> MVYSYTEKKRIRKDFGKRPQVLDVPYLLSIQLDSFQKFIEQDPEGQYGLEAAFRSVFPIQSYSGNSELQYVSYRLGEPVFDVQECQIRGVTYSAPLRVKLRLVIYEREAPEGTVKDIKEQEVYMGEIPLMTDNGTFVINGTERVIVSQLHRSPGVFFDSDKGKTHSSGKVLYNARIIPYRGSWLDFEFDPKDNLFVRIDRRRKLPATIILRALNYTTEQILDLFFEKVIFEIRDNKLQMELVPERLRGETASFDIEANGKVYVEKGRRITARHIRQLEKDDVKLIEVPVEYIAGKVVAKDYIDESTGELICAANMELSLDLLAKLSQSGHKRIETLFTNDLDHGPYISETLRVDPTNDRLSALVEIYRMMRPGEPPTREAAESLFENLFFSEDRYDLSAVGRMKFNRSLLREEIEGSGILSKDDIIDVMKKLIDIRNGKGEVDDIDHLGNRRIRSVGEMAENQFRVGLVRVERAVKERLSLGDLDTLMPQDMINAKPISAAVKEFFGS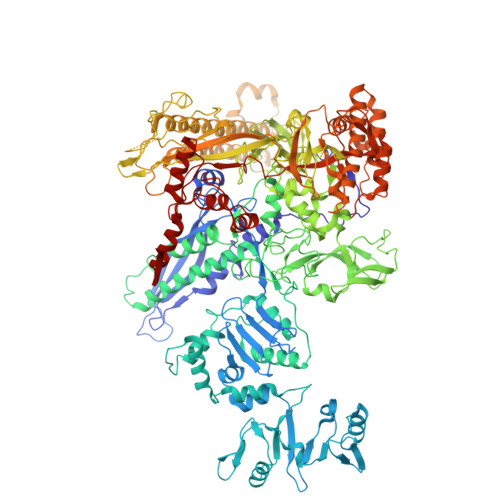SQLSQFMVQNNPLSEITHKRRISALGPGGLTRERAGFEVRDVHPTHYGRVCPIETPEGPNIGLINSLSVYAQTNEYGFLETPYRKVTDGVVTDEIHYLSAIEEGNYVIAQANSNLDEEGHFVEDLVTCRSKGESSLFSRDQVDYMDVSTQQVVSVGASLIPFLEHDDANRALMGANMQRQAVPTLRADKPLVGTGMERAVAVDSGVTAVAKRGGVVQYVDASRIVIKVNEDEMYPGEAGIDIYNLTKYTRSNQNTCINQMPCVSLGEPVERGDVLADGPSTDLGELALGQNMRVAFMPWNGYNFEDSILVSERVVQEDRFTTIHIQELACVSRDTKLGPEEITADIPNVGEAALSKLDESGIVYIGAEVTGGDILVGKVTPKGETQLTPEEKLLRAIFGEKASDVKDSSLRVPNGVSGTVIDVQVFTRDGVEKDKRALEIEEMQLKQAKKDLSEELQILEAGLFSRIRAVLVAGGVEAEKLDKLPRDRWLELGLTDEEKQNQLEQLAEQYDELKHEFEKKLEAKRRKITQGDDLAPGVLKIVKVYLAVKRRIQPGDKMAGRHGNKGVISKINPIEDMPYDENGTPVDIVLNPLGVPSRMNIGQILETHLGMAAKGIGDKINAMLKQQQEVAKLREFIQRAYDLGADVRQKVDLSTFSDEEVMRLAENLRKGMPIATPVFDGAKEAEIKELLKLGDLPTSGQIRLYDGRTGEQFERPVTVGYMYMLKLNHLVDDKMHARSTGSYSLVTQQPLGGKAQFGGQRFGEMEVWALEAYGAAYTLQEMLTVKSDDVNGRTKMYKNIVDGNHQMEPGMPESFNVLLKEIRSLGINIELEDE> MNDNYQNNYVVGRGTVYFDRFQDGTNRKTGEMYFGNTPEFTINTDSETLDHYSSDHGMRVMDASVLLEASQGGTFTCDNINADNLALWFLGEVSNTTQTQQTDAKEVFNPIMRGRYYQLGTTDDNPTGVRGVTNFQMVKADASIAISVGSGDITSIVGATVVNPAGNYEIDLEAGRIYIEPDSTDLSGNVQIAVQYDVDAQKRTLVIGKSNMVYGALRMISDNPVGLNKNYYFPKVSIAPDGDYALKGDDWQVMSFTFKAMQLNNIT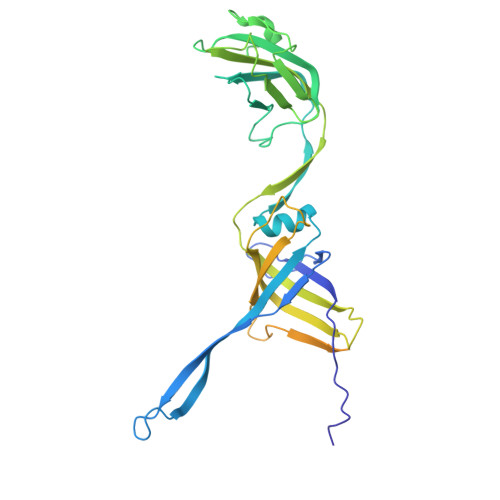QRVYIDIVEAAAAVDPTAQRTIEITPASTTATTGGAGVVCTVTVRDGTGTAVQGDAVTFTTVAGATVTPNSATTGATGTATTTVNRAAAGTATVTATLANGKAATTGTITFSAP>KPKLLNKFDKTIKAELDAAEKLRKRGKIEEAVNAFKELV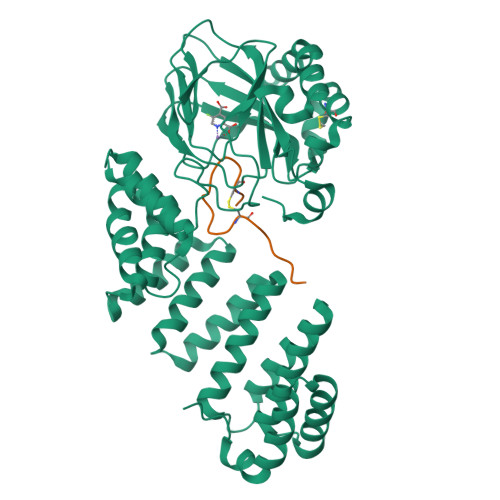RKYPQSPRARYGKAQCEDDLAEKRRSNEVLRGAIETYQEVASLPDVPADLLKLSLKRRSDRQQFLGHMRGSLLTLQRLVQLFPNDTSLKNDLGVGYLLIGDNDNAKKVYEEVLSVTPNDGFAKVHYGFILKAQNKIAESIPYLKEGIESGDPGTDDGRFYFHLGDAMQRVGNKEAYKWYELGHKRGHFASVWQRSLYNVNGLKAQPWWTPKETGYTELVKSLERNWKLIRDEGLAVMDKAKGLFLPEDENLREKGDWSQFTLWQQGRRNENACKGAPKTCTLLEKFPETTGCRRGQIKYSIMHPGTHVWPHTGPTNCRLRMHLGLVIPKEGCKIRCANETKTWEEGKVLIFDDSFEHEVWQDASSFRLIFIVDVWHPELTPQQRRSLPAI[2x];> DGDQSETSPSQNQGKCKDGLGEYTCTSLEGFEGKNSELF(1S,3R,4S,5S,7S)-4-{[2-(4-METHOXYPHENOXY)-2-METHYLPROPANOYL]AMINO}ADAMANTANE-1-CARBOXAMIDE 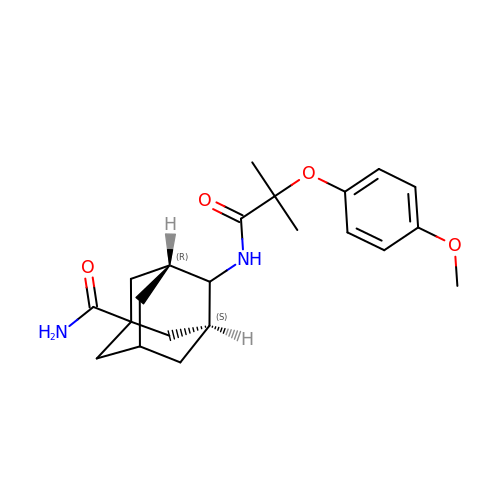| C22 H30 N2 O4 | MNVKIDPRYUGTTG-YINOZDTMSA-N>[2x]METLGGFPVEFLIQVTRLSKILMIKKEHIKKLRE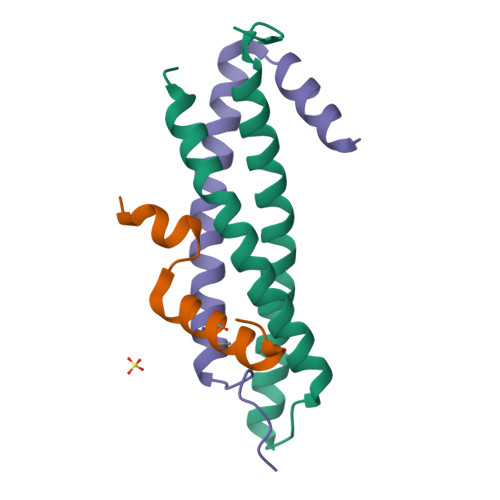MNTEAEKLKSYSMPISIEFQRRYATIVLELEQLNKDLNKVLHKVQQYCYELAPDQGLQPADQPTDMRRRCEEEAQEIVRHANSST;>GEFSSPPKWMAEIERDDIDMLKELGSLTTANLMEKVRGLQNLAYQLGLDESREMTRGKFLNILEKPKK[2x];>[2x]APMSSAWKTVACGGTRDQLFMQEKARQLLGRL> ERSASYKPVFVTEITDDLHFYVQDVETGTQLEKLMENMRNDIASHPPVEGSYAPRRGEFCIAKFVDGEWYRARVEK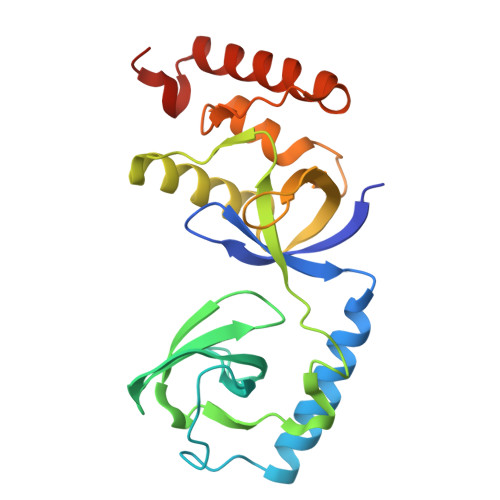VESPAKIHVFYIDYGNREVLPSTRLGTLSPAFSTRVLPAQATEYAFAFIQVPQDDDARTDAVDSVVRDIQNTQCLLNVEHLSAGCPHVTLQFADSKGDVGLGLVKEGLVMVEVRKEKQFQKVITEYLNAQESAKSARLNLWRYGDFRA The lectin pathway of complement is activated by complexes comprising a recognition component (mannose-binding lectin, serum ficolins, collectin-LK or collectin-K1) and a serine protease (MASP-1 or MASP-2). MASP-1 activates MASP-2, and MASP-2 cleaves C4 and C4b-bound C2. MASPs are homodimers that circulate as zymogens bound to the collagenous domains of MBL. Each MASP comprises two N-terminal CUB (C1r/C1s, Uegf, and bone morphogenetic protein-1) domains separated by an epidermal growth factor (EGF)-like domain followed by two short complement regulator (SCR) domains and a C-terminal serine protease (SP) domain.

In particular, MASP-2 CUB1-EGF-CUB2 (subsequently called MASP-2 3D) was crystallized in the presence of citrate that chelates Ca2+, and although Ca2+ was bound to the EGF-like domain, the CUB1 and CUB2 domains lacked Ca2+ and became partially disordered as a result (Feinberg et al., 2003). Because there was no structure of rat MASP-1 3D, and the existing structure of rat MASP-2 3D lacked two of the three Ca2+, including those Ca2+ that form part of the binding site for MBL, both rat MASP-1 3D and MASP-2 3D were crystallized in the presence of 2 mM calcium and diffraction data were collected. This resulted in one MASP-1 structure at 3.7 Å resolution and three independent MASP-2 structures at 2.6–2.7 Å resolution. For MASP-2 3D, 279 of 280 residues were visible. Interestingly, the three structures overlaid closely, with RMSDs of 0.682, 0.871, and 0.992 Å over 276 Cα atoms. The only notable differences were in the N-terminal seven residues and in a loop within the EGF-like domain (Thr125–Ser130), probably reflecting flexibility. A major difference, however, was that the structures now contained three bound Ca2+ compared with the single Ca2+ in the EGF-like domain of the earlier MASP-2 3D structure. In the MASP-2 CUB1 domain, Ca2+ formed contacts with six oxygen atoms in the side chains of Glu48, Asp56, Asp101, and Asn104 and the main chain oxygen of Ser103 (distances between 2.3 and 2.7 Å). In the MASP-2 CUB2 domain, Ca2+ formed contacts with five oxygen atoms at the side chains of Glu215, Asp225, Asp262, and Ser264. The firm identification in this study of the three Ca2+ sites in rat MASP-2 now resolves a key ambiguity of the earlier rat MASP-2 structure (Feinberg et al., 2003).

> KWPEPVFGRLVSPGFPEKYGNHQDRSWTLTAPPGFRLRLYFTHFNLELSYRCEYDFVKLTSGTKVLATLCGQESTDTERAPGNDTFYSLGPSLKVTFHSDYSNEKPFTGFEAFYAAEDVDECRTSLGDSVPCDHYCHNYLGGYYCSCRVGYILHQNKHTCSALCSGQVFTGRSGFLSSPEYPQPYPKLSSCAYNIRLEEGFSITLDFVESFDVEMHPEAQCPYDSLKIQTDKREYGPFCGKTLPPRIETDSNKVTITFTTDESGNHTGWKIHYTSTA Altogether CD38 appears to be a key player in the biosynthesis of calcium messengers which are involved in a wide range of cellular functions. Thus, the catalytic transformation of NAD+ involves the formation, via a ribooxocarbenium ion-like transition state, of a unique reaction intermediate that partitions between several competing pathways such as an irreversible hydrolytic process leading to ADP-ribose and a reversible minor pathway that governs the formation of cADPR. The L-shaped structure of bCD38 consists of two distinct domains separated by a cleft and connected by a hinge region. α-Helices are found mainly in the N-terminal and membrane-proximal domain of this transmembrane protein, whereas β-sheets are preponderant in the distal C-terminal domain. The active site of bCD38 consists in a funnel-shaped cavity with a fairly rigid structure; it buries the NMN+ moiety of the substrate and its scissile bond in its deepest non-polar and least solvent accessible region, whereas the AMP moiety interacts with its more solvent-exposed region, at the entrance of the catalytic cleft.

In agreement with observations on hCD38, incubation of crystals of wt bCD38 with rFNAD and aFNAD resulted in stable covalent intermediates whose structures could be resolved at high resolution. In both complexes, residue Glu218 was found covalently linked to the anomeric carbon C1′ of the fluorinated-ribose ring in an axial (α-anomeric) configuration. As in the Michaelis complex, the 2′-fluorine atom of rFNAD interacts with a conserved structural water molecule that is hydrogen bonded by the carbonyl and amide nitrogen backbone groups from residues Val116 and Leu137 respectively. Thus, although both copies of the enzyme contains a covalent adduct formed by reaction between the carboxylate of Glu218 and the C1′ of the N-ribose of rFNAD, the conformation of the covalently bound intermediates are quite different. In one copy of the enzyme (chain B), we were able to model the complete ADP-2′-deoxy-2′-fluororibosyl moiety in a folded conformation with the adenine ring stacked at full occupancy against Trp181. In the second copy of the enzyme (chain A), we were only able to model the 2′-deoxy-2′-fluororibose-diphosphate moiety of the covalently bound adduct. When the complete ligand could be observed it was found to adopt a ‘folded’ conformation. In contrast to the more extended conformation observed in the Michaelis complex with rFNAD where the adenine ring stacked against Trp168 (see above), through rotations around its C4′–C5′ and C5′–O5′ bonds the adenosine moiety has flipped over and the adenine ring is now stacked against residue Trp181, a position close to that previously occupied by the nicotinamide ring in the active site in the non-covalent Michaelis complex.

>[2x]YKWHYSGLNRWHGAGSTADFQKIIQERCDTYTQTIRPGSRSRNCQAIRQAFMSAFISKDPCKATKEDYNSLINLAPPTVPCGQQVFWSKTKELAHEYAKRRRLMTLEDTLLGYLADGLRWCGEPGSSDLNIWSCPDWRKDCRTNYLSVFWEVLSERFAESACNTVRVVLNGSLENAFDSMSIFGRVEAPNLRPQVELEAWLVHDTGKPPSDSCSGSSIRKLKSILDGRNVKFRCMDNLSRDQFLQRS> MAARLLAPPGPDSFKPFTPESLANIERRIAESKLKKPPKADGSHREDDEDSKPKPNSDLEAG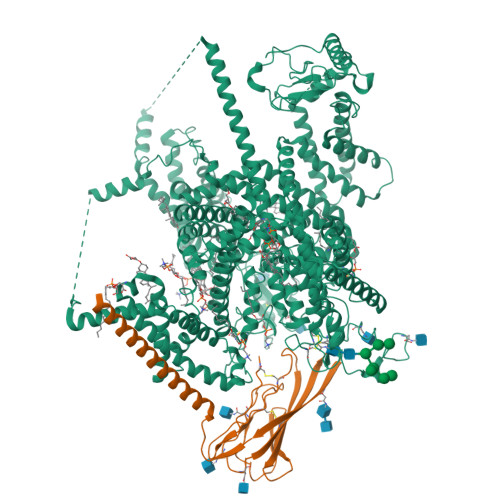KSLPFIYGDIPQGLVAVPLEDFDPYYLTQKTFVVLNRGKTLFRFSATPALYILSPFNLIRRIAIKILIHSVFSMIIMCTILTNCVFMTFSNPPDWSKNVEYTFTGIYTFESLVKIIARGFCIDGFTFLRDPWNWLDFSVIMMAYITEFVNLGNVSALRTFRVLRALKTISVIPGLKTIVGALIQSVKKLSDVMILTVFCLSVFALIGLQLFMGNLRNKCVVWPINFNESYLENGTKGFDWEEYINNKTNFYTVPGMLEPLLCGNSSDAGQCPEGYQCMKAGRNPNYGYTSFDTFSWAFLALFRLMTQDYWENLYQLTLRAAGKTYMIFFVLVIFVGSFYLVNLILAVVAMAYEEQNQATLEEAEQKEAEFKAMLEQLKKQQEEAQAAAMATSAGTVSEDAIEEEGEEGGGSPRSSSEISKLSSKSAKERRNRRKKRKQKELSEGEEKGDPEKVFKSESEDGMRRKAFRLPDNRIGRKFSIMNQSLLSIPGSPFLSRHNSKSSIFSFRGPGRFRDPGSENEFADDEHSTVEESEGRRDSLFIPIRARERRSSYSGYSGYSQGSRSSRIFPSLRRSVKRNSTVDCNGVVSLIGGPGSHIGGRLLPEATTEVEIKKKGPGSLLVSMDQLASYGRKDRINSIMSVVTNTLVEELEESQRKCPPCWYKFANTFLIWECHPYWIKLKEIVNLIVMDPFVDLAITICIVLNTLFMAMEHHPMTPQFEHVLAVGNLVFTGIFTAEMFLKLIAMDPYYYFQEGWNIFDGFIVSLSLMELSLADVEGLSVLRSFRLLRVFKLAKSWPTLNMLIKIIGNSVGALGNLTLVLAIIVFIFAVVGMQLFGKSYKECVCKINQDCELPRWHMHDFFHSFLIVFRVLCGEWIETMWDCMEVAGQAMCLIVFMMVMVIGNLVVLNLFLALLLSSFSADNLAATDDDGEMNNLQISVIRIKKGVAWTKLKVHAFMQAHFKQREADEVKPLDELYEKKANCIANHTGADIHRNGDFQKNGNGTTSGIGSSVEKYIIDEDHMSFINNPNLTVRVPIAVGESDFENLNTEDVSSESDPEGSKDKLDDTSSSEGSTIDIKPEVEEVPVEQPEEYLDPDACFTEGCVQRFKCCQVNIEEGLGKSWWILRKTCFLIVEHNWFETFIIFMILLSSGALAFEDIYIEQRKTIRTILEYADKVFTYIFILEMLLKWTAYGFVKFFTNAWCWLDFLIVAVSLVSLIANALGYSELGAIKSLRTLRALRPLRALSRFEGMRVVVNALVGAIPSIMNVLLVCLIFWLIFSIMGVNLFAGKYHYCFNETSEIRFEIEDVNNKTECEKLMEGNNTEIRWKNVKINFDNVGAGYLALLQVATFKGWMDIMYAAVDSRKPDEQPKYEDNIYMYIYFVIFIIFGSFFTLNLFIGVIIDNFNQQKKKFGGQDIFMTEEQKKYYNAMKKLGSKKPQKPIPRPLNKIQGIVFDFVTQQAFDIVIMMLICLNMVTMMVETDTQSKQMENILYWINLVFVIFFTCECVLKMFALRHYYFTIGWNIFDFVVVILSIVGMFLADIIEKYFVSPTLFRVIRLARIGRILRLIKGAKGIRTLLFALMMSLPALFNIGLLLFLVMFIFSIFGMSNFAYVKHEAGIDDMFNFETFGNSMICLFQITTSAGWDGLLLPILNRPPDCSLDKEHPGSGFKGDCGNPSVGIFFFVSYIIISFLIVVNMYIAIILENFSVATEESADPLSEDDFETFYEIWEKFDPDATQFIEYCKLADFADALEHPLRVPKPNTIELIAMDLPMVSGDRIHCLDILFAFTKRVLGDSGELDILRQQMEERFVASNPSKVSYEPITTTLRRKQEEVSAVVLQRAYRGHLARRGFICKKTTSNKLENGGTHREKKESTPSTASLPSYDSVTKPEKEKQQRAEEGRRERAKRQKEVRESKC;> MGRLLALVVGAALVSSACGGCVEVDSETEAVYGMTFKILCISCKRRSETNAETFTEWTFRQKGTEEFVKILRYENEVLQLEEDERFEGRVVWNGSRGTKDLQDLSIFITNVTYNHSGDYECHVYRLLFFENYEHNTSVVKKIHIEVVDKANRDMASIVSEIMMYVLIVVLTIWLVAEMIYCYKKIAAATETAAQENASEYLAITSESKENCTGVQVAE>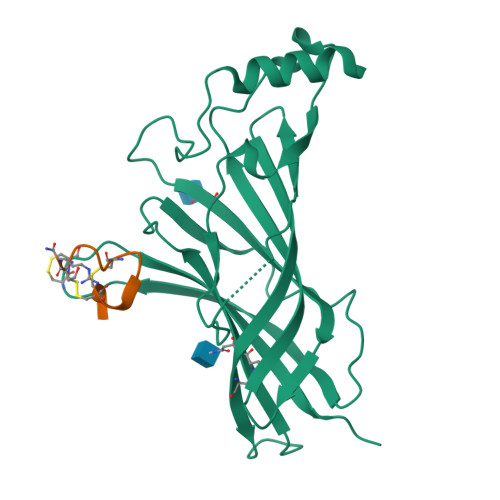 ADGKYAQKLFNDLFEDYSNALRPVEDTDKVLNVTLQITLSQIKDMDERNQILTAYLWIRQIWHDAYLTWDRDQYDGLDSIRIPSDLVWRPDIVLYNKADDESSEPVNTNVVLRYDGLITWDAPAITKSSCVVDVTYFPFDNQQCNLTFGSWTYNGNQVDIFNALDSGDLSDFIEDVEWEVHGMPAVKNVISYGCCSEPYPDVTFTLLLKRRSHHHHHH;> GCCSDPRCRYRCR>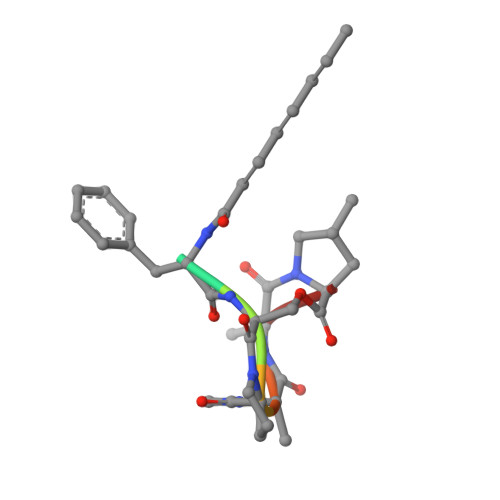 XFSPAAP>[2x]MNLKDKILGVAKELFIKNGYNATTT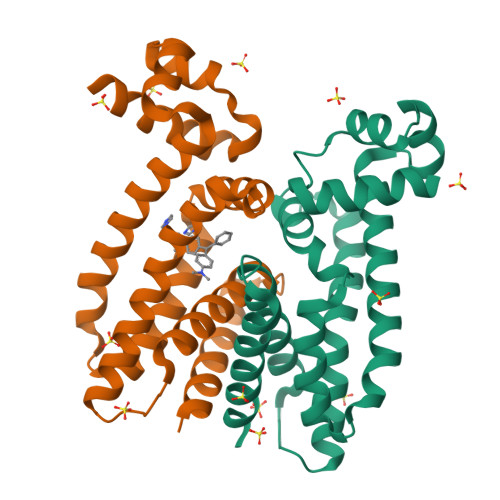GEIVKLSESSKGNLYYHFKTKENLFLEILNIEESKWQEQWKSEQIKAKTNREKFYLYNELSLTTEYYYPLQNAIIEFYTEYYKTNSINEKMNKLQNKYIDAYHVIFKEGNLNGEWSINDVNAVSKIAANAVNGIVTFTHEQNINERIKLMNKFSQIFLNGLSKHHHHHH> MSADNGLIIGIDLGTTNSCVSVMEGGRPVVLENPEGKRTTPSIVSYKNNEIIVGDAAKRQMVTNPNTIVSIKRLMGTSNKVKVQNADGTTKELSPEQVSAQILSYLKDFAEKKIGKKISRAVITVPA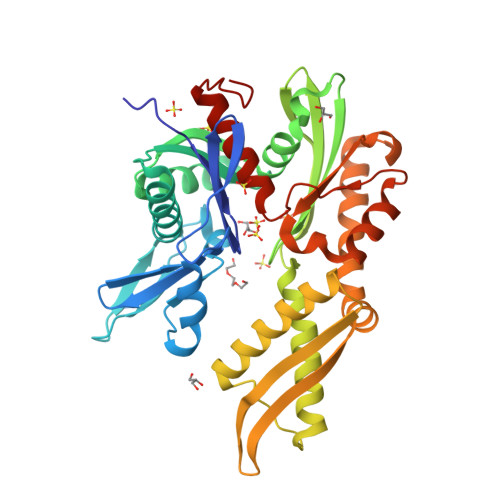YFNDAERNATKTAGKIAGLNVERIINEPTAAALAYGIDKASREMKVLVYDLGGGTFDVSLLDIAEGTFEVLATAGDNRLGGDDWDNKIIEYISAYIAKEHQGKNLSKDKMAMQRLKEAAERAKIELSAQLETIISLPFLTVTQKGPVNVELKLTRAKFEELTKPLLERTRNPISDVIKEAKIKPEEINEILLVGGSTRMPAVQKLVESMVPGKKPNRSINPDEVVAIGAAIQGGVLRGDLEHHHHHH>[2x]RSRLVQFQKNTDEPMGITLKMNELNHCIVARIMHGGMIHRQGTLHVGDEIREINGI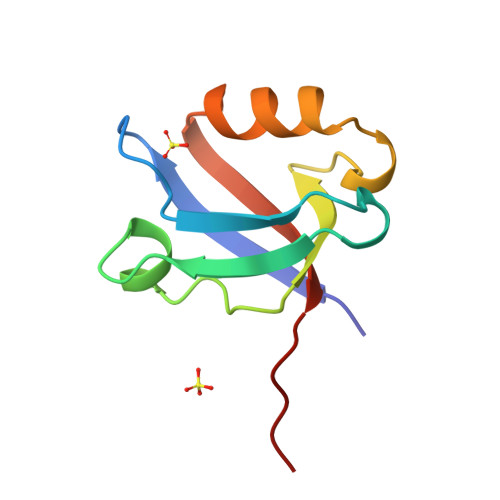SVANQTVEQLQKMLREMRGSITFKIVPSYREF>[2x]GSHMASMTAVHAGNINFKWDPKSLEIRTLAVERLLEPLVTQVTTLVNTNSKGPSNKKRGRSKKAHVLAASVEQATENFLEKGDKIAKESQFLKEELVVAVEDVRKQGDLMKSAAGEFADDPCSSVKRGNMVRAARALLSAVTRLLILADMADVYKLLVQLKVVEDGILKLRNAGNEQDLGIQYKALKPEVDKLNIMAAKRQQELKDVGNRDQMAAARGILQKNVPILYTASQACLQHPDVAAYKANRDLIYKQLQQAVTGISNAAQATASDDAAQHQGGSGGELAYALNNFDKQIIVDPLSFSEERFRPSLEERLESIISGAALMADSSCTRDDRRERIVAECNAVRQALQDLLSEYMGNAGRKERSDALNSAIDKMTKKTRDLRRQ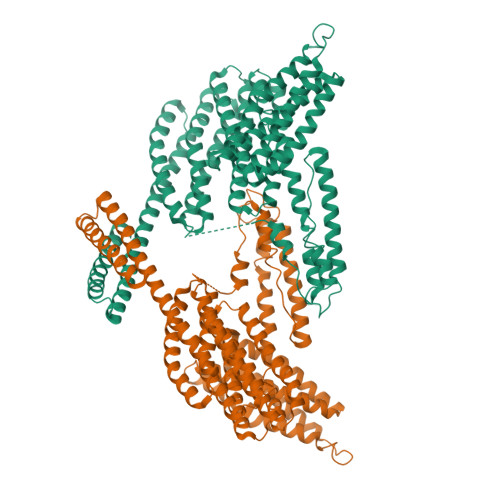LRKAVMDHVSDSFLETNVPLLVLIEAAKNGNEKEVKEYAQVFREHANKLIEVANLACSISNNEEGVKLVRMSASQLEALCPQVINAALALAAKPQSKLAQENMDLFKEQWEKQVRVLTDAVDDITSIDDFLAVSENHILEDVNKCVIALQEKDVDGLDRTAGAIRGRAARVIHVVTSEMDNYEPGVYTEKVLEATKLLSNTVMPRFTEQVEAAVEALSSDPAQPMDENEFIDASRLVYDGIRDIRKAVLMIRTPEELDDSDFETEDFDVRSRTSVQTEDDQLIAGQSARAIMAQLPQEQKAKIAEQVASFQEEKSKLDAEVSKWDDSGNDIIVLAKQMCMIMMEMTDFTRGKGPLKNTSDVISAAKKIAEAGSRMDKLGRTIADHCPDSACKQDLLAYLQRIALYCHQLNICSKVKAEVQNLGGELVVSGVDSAMSLIQAAKNLMNAVVQTVKASYVASTKYQKSQGMASLNLPAVSWKMKAPEKKPLVKREKQDETQTKIKRASQKKHVNPVQALSEFKAMDSI> CPVNWVEHERSCYWFSRSGKAWADADNYCRLEDAHLVVVTSWEEQKFVQHHIGPVNTWMGLHDQNGPWKWVDGTDYETGFKNWRPEQPDDWYGHG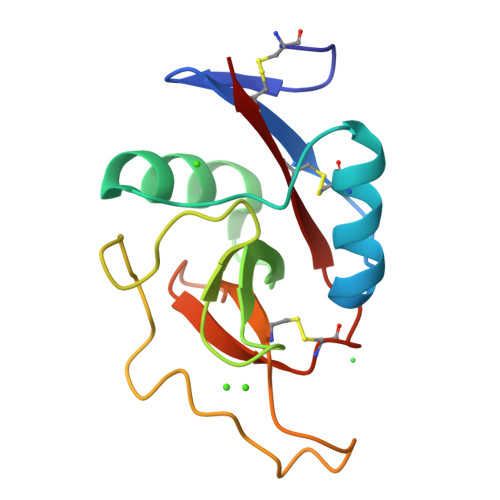LGGGEDCAHFTDDGRWNDDVCQRPYRWVCETEL> MTKFSGNELRAELYRRAFLSYSVAPGALGMFGRSLLAKGARAEALANGTVMSGSHWGVFTATVENGRATAFTPWEKDPHPSPMLAGVLDSIYSPTRIKYPMVRREFLEKGVNADRSTRGNGDFVRVSWDQALDLVAAEVKRVEETYGPQGVFGGSYGWKSPGRLHNCTTLLRRMLTLAGGYVNGAGDYSTGAAQVIMPHVVGTLEVYEQQTAWPVLAENTEVMVFWAADPIKTSQIGWVIPEHGAYPGLEALKAKGTKVIVIDPVRTKTVEFFGAEHITPKPQTDVAIMLGMAHTLVAEDLYDKDFIANYTSGFDKFLPYLDGETDSTPKTAEWAEGISGVPAETIKELARLFESKRTMLAAGWSMQRMHHGEQAHWMLVTLASMLGQIGLPGGGFGLSYHYSGGGTPSTSGPALAGITDGGAATKGPEWLAASGASVIPVARVVDMLENPGAEFDFNGTRSKFPDVKMAYWVGGNPFVHHQDRNRMVKAWEKLETFVVHDFQWTPTARHADIVLPATTSYERNDIETIGDYSNTGILAMKKIVEPLYEARSDYDIFAAVAERLGKGKEFTEGKDEMGWIKSFYDDAAKQGKAAGVEMPAFDAFWAEGIVEFPVTDGADFVRYASFREDPLLNPLGTPTGLIEIYSKNIEKMGYDDCPAHPTWMEPLERLDGPGAKYPLHIAASHPFNRLHSQLNGTVLR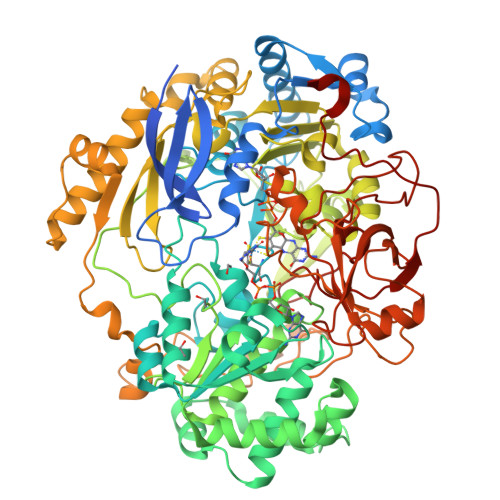EGYAVQGHEPCLMHPDDAAARGIADGDVVRVHNDRGQILTGVKVTDAVMKGVIQIYEGGWYDPSDVTEPGTLDKYGDVNVLSADIGTSKLAQGNCGQTVLAEVEKYTGPAVTLTGFVAPKAAE>[2x]MAILAFQKPENVLMMETSDSIAKFEFKPLEPGYGITIGNALRRILLSSLEGFAITAIKIEGVEHEFATIPGVLEDVTNIILNLKQVRFKQIVPNADVEKATIVISNSEVFRAGDLNAQLSNFEVLNSNLVICHLDKSATLTMEFSINKGRGYVSAEENRAEHNELSTIAIDSIYTPIRNVKYAVENFRVEQKTDYEKLLMEVTTDGSIRPVDALREAAQILISHFSLFAENKIAIEYVDIVDTDEFDEDSLHMRQLLKSKLSGLDLSVRALNCLNAAGVDTLGDLVSLSRSDLMKIRNFGKKSLTELDELLATLNLSFGMDISKYKLDKD;> MTPTTNNKRINFASIKNPLFYPDFLEVQLKSFHDFLQLDTPPERRKKEGLYKVFAENFPITDTRNNFVLEFLDYYIDPPKYSIEECLSRGLTYSVPLKAKLKLYCTDPDHEDFATVIQDVFLGPIPYMTSSGTFVINGAERVIVSQLHRSPGVFFGQSLHTNGTKLYSARIIPFKGSWIEFATDINNVMYAYIDRKKKLPVTTLLRAIGFEADKDILDIFNLADEVKVTKANLKKCIGRKLAARVINTYIDDLSDEDTGEVVSMERITVVVDREVELTEDNIEAILNSNAQTILLHRNDSNTSDYSIIFNTLQKDPCNSEKEALYYVYRQLRNAEPADDASAREVITNLFFSDKRYDLGDVGRYRINKKLNLNIDPDIKVLTNEDIIEIIKYLIELVNSKASVDDIDHLSNRRVRTVGEQLYNQFGIGLARMARTVRDRMNVRDNEVFTPIDLVNAKTISSVVNSFFGTNALSQFMDQTNPLAEITHKRRLSALGPGGLSRERAGFEVRDVHYTHYGRLCPIETPEGPNIGLISSLCVYAKISDLGFITTPYREVKNGKVDFSDNGLKYYTAEEEEEKTVAQGNAPLDENGRFVRERVKARYESDFPLVTPDEVDLMDVSPTQIASIAAALIPFLEHDDANRALMGSNMMRQAVPLLRPESPIVGTGIEGKLVKDSRTQIVAERGGEVVFVDASCIKIRYDRTADEEFVSFDDAIVTYYLPKYRKTNQSTTIDLHPICSKGDRVEAGQILTEGYSTQGGELALGRNVQVAYMPWKGYNYEDAIVLNERMVREDFFTSVHVDEYILEVRETKRGLEELTSDIPNVSEDATRDLDENGIVRIGAHIEPGDILIGKITPKGESDPTPEEKLLRAIFGDKAGDVKDASLKATPSLRGVVIDTKLFSKAAKKKSRTSTKEAVSKLDETYAKRQQQLHERLIEKLTELTKGKTCCGVKDYLNVELIKAGSKFTKKDLEALDFNVIQLSDWTNDAHTNELIKAVAVNYLKHSKEIEAELRRRKLDETIGDELPAGIVQMAKVYIAKKRKIQVGDKMAGRHGN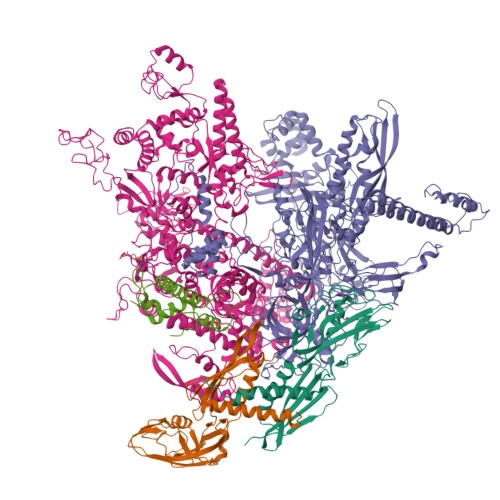KGIVSKIVRQEDMPFLADGTPVDICLNPLGVPSRMNLGQIFEAVLAWAGRKMNVKFATPIFDGASLNDMNEWTDKAGLPRDGKTYLYDGGTGERFDQPATVGVTYFLKLGHMVDDKMHARSIGPYSLITQQPLGGKAQFGGQRFGEMEVWALEAFGASHILQEILTVKSDDVVGRSKAYEAIVKGDPMPTPGIPESLNVLLHELKGLGLSFSLD;> MAFRKENKIKNNFSKIRITLASPEEILENSFGEVLKPETINYRTYKPERDGLFCERIFGPVKDFECHCGKYKRIRYRGIVCDRCGVEVTEKKVRRERMGHIHLVVPVAHIWYFRSLPNKIGYLLGLPTKKLDAIIYYERYVVIQPGVAEGLSQLDLLSEEEYLDKLDEIERTHKGNQNLEDTNPDKFIAKIGAEAIYDLLCRVDLDSISYELRDRANTDGSQQRKTEALKRLQVVESFRASKGVNRPEWMVMKVIPVIPPDLRPLVPLDGGRFATSDLNDLYRRVIIRNNRLKRLIEIKAPEVILRNEKRMLQEAVDSLFDNSRKSSAVKSDNNRPLKSLSDSLKGKQGRFRQNLLGKRVDYSARSVIVVGPELKMHECGLPKDMAAELYKPFIIRKLIERGIVKTVKSAKKIVDRKEPVIWDILEYVMKGHPVLLNRAPTLHRLGIQAFQPKLIEGKAIQLHPLSCTAFNADFDGDQMAVHLPLSNEAILEAQLLMLASHNILNPANGAPITVPSQDMVLGLYYITKLRPNTKGHGLIFYGPEEATIAYNEGKVDIHAPIKVYVEDYENGELVRRMVETSVGRLMVNEYVPKKVGYVNEVLGKKALRDIIGSVIKICGVATTAKFLDDIKNLGYYMAFKGGLSFNLADVLIPDEKDQLIQEGYTAVEQIMQDYSMGFITFNERYNQIIDTWTHINGRLSNVLIKQLSSDNDGFNSVFMMMDSGARGSKEQIRQLSGMRGLMAKPQKSGAEGGQIIENPILSNFKEGLSVLEYFISTHGARKGLADTALKTADAGYLTRRLVDVSHDVIITEEDCGTLRGLLTTELKQNEDVVASLYERILGRVSVHDIIHPTTGDIIVRAGEEIREQAAQIIEDSPIEAVEIRSVLTCESKKGVCAKCYGRNLATNRMVQRGEVVGVIAAQSIGEPGTQLTLRTFHVGGIASNVATENSLLSKYDGILEFEELRAVDATDESHQVVVSRMTELRIADPNTGIILANHNIPYGAKLFFRQGDAVKKGDKIIEWDPFNAVIVSEVAGTLSFEGVVENVTFKMESDETTGLKEKIIIESKDKTMAPYARIIDENGEMLKNYSLPMGAHVVKDDGDTVKVGEILVKIPRSVGKAGDITGGLPRVTELFEARNPSNPAIVSEIDGEIGFGKLKRGNREITVTSKLGEEKKYLIPLSKQLLVQENDFVRAGTPLSDGAITPADILAIKGPTAVQEYIVNEVQDVYRLQGVKINDKHFEVIVRQMMRKVEIVDPGDTLFLEQQVVDKFEVMEENDRIWGKKVVIDAGDSQVLKAGQIVTARKLRDENSMLKRKDLKIVKVRDAKSATASQILQGITRAALQTKSFMSAASFQETTKVLNEAAICGKTDYLEGLKENVICGHLIPAGTGLRDYEKLVVMHRDDYEKATAERKSFLSEPTAEPAMEEAPSEHHHHHH;> MELKKMNVPMDTITRDMVRLSEDTENVYETVMIIAKRANQIGQQMKQDLEKKLQDFSSSNDNLEEVFENREQIEISRYYEHLPKPGLIATAEYEQDKLYHRMPGATSTND>MENDMSSNQTLAEKKIPVS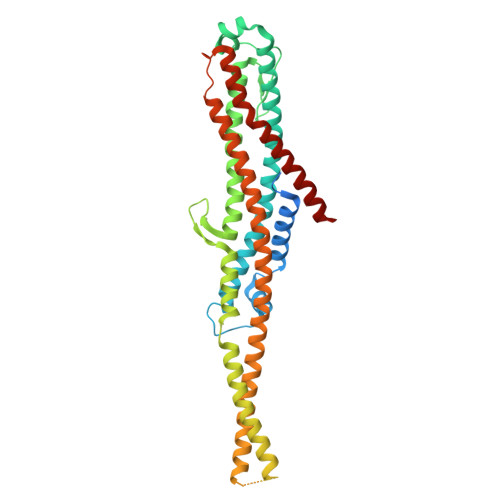EVPSATLKMLTSQAEGVARPGGIFTKGDLINIKLYVKHSLELPFTLEGVKEYIGYNDIDIDGLKPAKMATLFKEIHDHALSWSGVESKVQQQSIDLENAGKQITLTGDEIISVIDQMPIIERVKNKLGDLTDKQLAEITYTNDDKEIAVELGNILESMKKDIKRQQENTQKVKTAVSDFKLKLIGGELSDGTIAQGLQPQISSKKKLMDDNNLSTTIKDLQSKIDEKNKEIDQFQKDYNKYVGLAFSGMVGGIISWAITGGIFGDKAEKARKQKNKLIDEVKDLQSQVKDKSALQTSVQNLSLSFAGIHTSMVDAEEALNHLDFMWNTMLTQITTSRDKFDDINDALKLTSFVIAFKQVIEPWRDVQGSAAQLIQTFDEALAEYKKLYH[2x]> GLNHMLKIGSHVSMSGKKMLLAASEEAASYGANTFMIYTGAPQNTKRKSIEELNIEAGRQHMQAHGIEEIVVHAPYIINIGNTTNLDTFSLGVDFLRAEIERTEAIGAKQLVLHPGAHVGAGVEAGLRQIIRGLNEVLTREQNVQIALETMAGKGSECGRTFEELAYIIDGVAYNDKLSVCFDTCHTHDAGYDIVNDFDGVLEEFDRIIGLGRLKVLHINDSKNPRGSRKDRHENIGFGHIGFAALNYIVHHPQLEDIPKILETPYVGE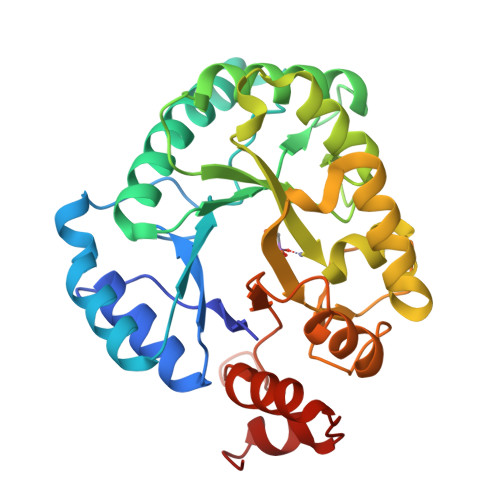DKNNKKPPYKHEIAMLRAQSFDDQLLEKINAGAE>EFATMEAFEISDFKEHAKKKSMWAGALNKVTISGLMGVFTEDEDLMALPIHRDHCPALLKIFDEIIVNATDHERACHNKTKKVTYIKISFDKGVFSCENDGPGIPIAKHEQASLIAKRDVYVPEVASCHFLAGTNINKAKDCIKGGTNGVGLKLAMVHSQWAILTTADGAQKYVQHINQRLDIIEPPTITPSREMFTRIELMPVYQELGYAEPLSETEQADLSAWIYLRACQCAAYVGKGTTIYYNDKPCRTGSVMALAKMYTLLSAPNSTIHTATIKADAKPYSLHPLQVAAVVSPKFKKFEHVSVINGVNCVKGEHVTFLKKTINEMVVKKFQQTIKDKNRKTTLRDSCSNIFIVIVGSIPGIEWTGQRKDELSIAENVFKTHYSIPSSFLTSMTKSIVDILLQSISKKDNHKQVDVDKYTRARNAGGKRAQDCMLLAAEGDSALSLLRTGLTLGKSNPSGPSFDFCGMISLGGVIMNACKKVTNITTDSGETIMVRNEQLTNNKVLQGIVQVLGLDFNCHYKTQEERAKLRYGCIVACVDQDLDGCGKILGLLLAYFHLFWPQLIIHGFVKRLLTPLIRVYEKGKTMPVEFYYEQEFDAWAKKQTSLANHTVKYYKGLAAHDTHEVKSMFKHFDNMVYTFTLDDSAKELFHIYFGGESELRKRELCTGVVPLTETQTQSIHSVRRIPCSLHLQVDTKAYKLDAIERQIPNFLDGMTRARRKILAGGVKCFASNNRERKVFQFGGYVADHMFYHHGDMSLNTSIIKAAQYYPGSSHLYPVFIGIGSFGSRHLGGKDAGSPRYISVQLASEFIKTMFPAEDSWLLPYVFEDGQRAEPEYYVPVLPLAIMEYGANPSEGWKYTTWARQLEDILALVRAYVDKDNPKHELLHYAIKHKITILPLRPSNYNFKGHLKRFGQYYYSYGTYVISEQRNIITITELPLRVPTVAYIESIKKSSNRMTFIEEIIDYSSSETIEILVKLKPNSLNRIVEEFKETEEQDSIENFLRLRNCLHSHLNFVKPKGGIIEFNTYYEILYAWLPYRRELYQKRLMREHAVLKLRIIMETAIVRYINES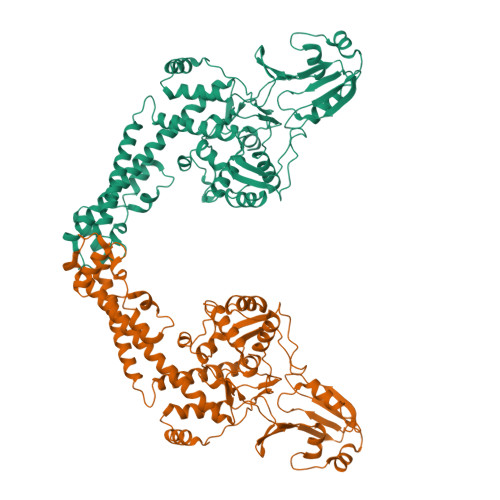AELNLSHYEDEKEASRILSEHGFPPLNHTLIISPEFASIEELNQKALQGCYTYILSLQARELLIAAKTRRVEKIKKMQARLDKVEQLLQESPFPGASVWLEEIDAVEKAIIKGRNTQWKFHENLYFQGHHHHHHHH[2x]>SNAMSKLQQILTYLESEKLDVAVVSDPVTINYLTGFYSDPHERQMFLFVLADQEPLLFVPALEVERASSTVSFPVVGYVDSENPWQKIKHALPQLDFKRVAVEFDNLILTKYHGLKTVFETAEFDNLTPRIQRMR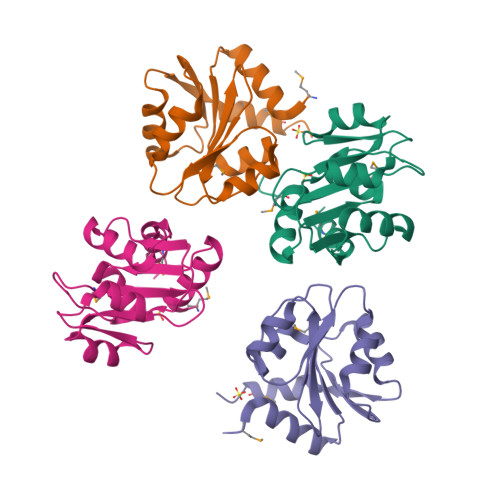LIK[4x]> TTSSQK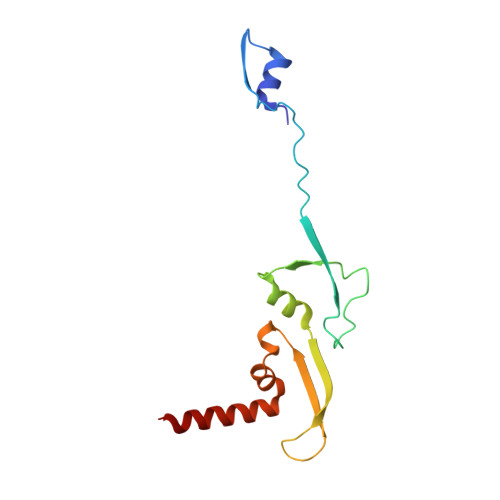FIARNRAPRVQIEYDVELYGAEKKVQLPFVMGVMADLAGKPAEPQAAVADRKFLEIDVDNFDARLKAMKPRVAFNVPNVLTGEGNLSLDITFESMDDFSPAAVARKVDSLNKLLEARTQLANLLTY> VWRKHYITYRINNYTPDMN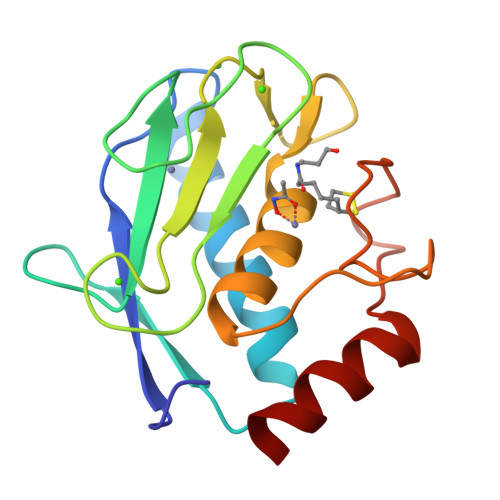REDVDYAIRKAFQVWSNVTPLKFSKINTGMADILVVFARGAHGDDHAFDGKGGILAHAFGPGSGIGGDAHFDEDEFWTTHSGGTNLFLTAVHEIGHSLGLGHSSDPKAVMFPTYKYVDINTFRLSADDIRGIQSLYG> MTGIPTVTARPWTQRPRAENSTTNPTYFFTFGDAYSQTGFSASGTQPSASNPMGNPDLGIGTTTNGPNWIGYLTT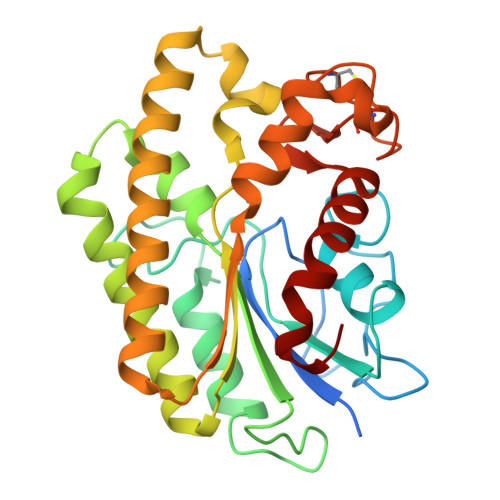TENASLVLSYNLAAGGATIDNALVPAYPGDLASQFRLFEDVYADKPASAPWSAEDAVFGVWIGINDIGNAYYSTDAETYTPKLISRLESLVEEVYKNGGRKFLFLNVPPTSRSPLFLEQGEEVVKQHAEYLSVYNENLEGMVDDFTKKKGDVTTVLYDSWSFMTKILDDPTAYGFPDATCINDDGTSCIWWNNYHPGMKYHLLQAEDMKPKLRKLGGW>[4x]MGSSHHHHHHSQDPMAPTTTMGSALYPLGEMRRSQRADGLAAVLAIGTANPPNCV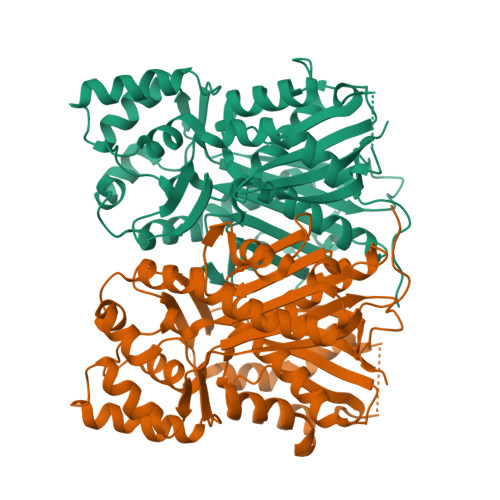TQEEIPDFYFRVTNSDHLTALKDKFKRICQEMGVQRRYLHHTEEMLSAHPEFVDRDAPSLDARLDIAADAVPELAAEAAKKAIAEWGRPAADITHLVVTTNSGAHVPGVDFRLVPLLGLRPSVRRTMLHLNGCFAGCAALRLAKDLAENSRGARVLVVAAELTLMYFTGPDEGCFRTLLVQGLFGDGAAAVIVGADADDVERPLFEIVSAAQTIIPESDHALNMRFTERRLDGVLGRQVPGLIGDNVERCLLDMFGPLLGGDGGGGWNDLFWAVHPGSSTIMDQVDAALGLEPGKLAASRRVLSDYGNMSGATVIFALDELRRQRKEAAAAGEWPELGVMMAFGPGMTVDAMLLHATSHVN One mechanism by which phages and other mobile genetic elements are able to overcome the CRISPR-Cas system is through the expression of anti-CRISPR proteins. We previously reported that gene 34 from Pseudomonas phage JBD5, which encodes the protein AcrE1, shows anti-CRISPR activity against the type I-E system of P. aeruginosa strain SMC4386 (4). We show that AcrE1 binds to the CRISPR-associated helicase/nuclease Cas3 and that the C-terminal region of the anti-CRISPR protein is important for its inhibitory activity. In summary, these experiments demonstrate that AcrE1 functions by blocking the activity of Cas3 without inhibiting the DNA-binding activity of Cascade.

(c) Structural overlay of the X-ray crystal structures of the AcrE1 proteins with an N-terminal (blue) and C-terminal (red) 6×His tag reveals virtually identical structures. Thus, the unusual nature of the C-terminal sheet was not a result of the presence of the 6×His affinity purification tag fused to the C terminus. The C-terminal β-sheet region is unusual because both sides of the sheet are exposed to solvent, contrasting with typical β-sheets, which pack a hydrophobic surface on one side against helices or other sheets. We also examined the packing of the C-terminal β-sheet within the crystal and observed no contacts that stabilize it in this position. Residues 82 to 90 form an antiparallel β-sheet that protrudes at a 90° angle from the end of helix 3. This sheet structure appears to be stabilized by multiple interactions between residues at the base of the sheet and residues in helices 1, 2, and 3. A salt bridge is formed between E41 and R89.

>[3x]HHHHHHMEKKLSDAQVALVAAWRKYPDLRESLEEAASILSLIVFQAETLSDQANELANYIRRQGLEEAEGACRNIDIMRAKWVEVCGEVNQHGIRVYGDAIDRDVD>[6x]MRLC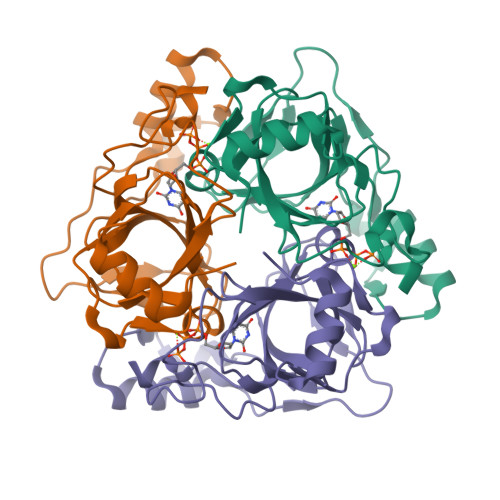DRDIEAWLDEGRLSINPRPPVERINGATVDVRLGNKFRTFRGHTAAFIDLSGPKDEVSAALDRVMSDEIVLDEGEAFYLHPGELALAVTLESVTLPADLVGWLDGRSSLARLGLMVHVTAHRIDPGWSGCIVLEFYNSGKLPLALRPGMLIGALSFEPLSGPAVRPYNRREDAKYRNQQGAVASRIDKD>MSDKLPYKVADIGLAAWGRK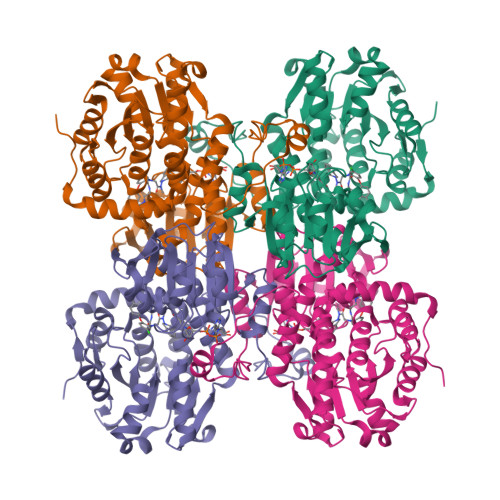ALDIAENEMPGLMRMRERYSASKPLKGARIAGCLHMTVETAVLIETLVTLGAEVQWSSCNIFSTQDHAAAAIAKAGIPVYAWKGETDEEYLWCIEQTLYFKDGPLNMILDDGGDLTNLIHTKYPQLLPGIRGISEETTTGVHNLYKMMANGILKVPAINVNDSVTKSKFDNLYGCRESLIDGIKRATDVMIAGKVAVVAGYGDVGKGCAQALRGFGARVIITEIDPINALQAAMEGYEVTTMDEACQEGNIFVTTTGCIDIILGRHFEQMKDDAIVCNIGHFDVEIDVKWLNENAVEKVNIKPQVDRYRLKNGRRIILLAEGRLVNLGCAMGHPSFVMSNSFTNQVMAQIELWTHPDKYPVGVHFLPKKLDEAVAEAHLGKLNVKLTKLTEKQAQYLGMSCDGPFKPDHYRY[2x]[(2~{S})-2-hexadecanoyloxy-3-[[(2~{R})-3-[[(2~{S})-3-[(5~{E},8~{E},11~{Z},14~{E})-icosa-5,8,11,14-tetraenoyl]oxy-2-[(9~{E},12~{Z})-octadeca-9,12-dienoyl]oxy-propoxy]-oxidanyl-phosphoryl]oxy-2-oxidanyl-propoxy]-oxidanyl-phosphoryl]oxy-propyl] 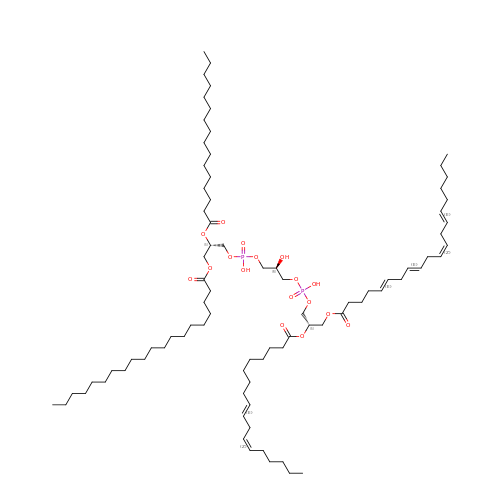icosanoate | C83 H150 O17 P2 | UOSHLVKGNDKXAL-XFYAQXJZSA-N1-[(1R)-3-(6-{[(BENZYLAMINO)CARBONYL]AMINO}-1H-INDOL-1-YL)-1-(HYDROXYMETHYL)PROPYL]-1H-IMIDAZOLE-4-CARBOXAMIDE | C24 H26 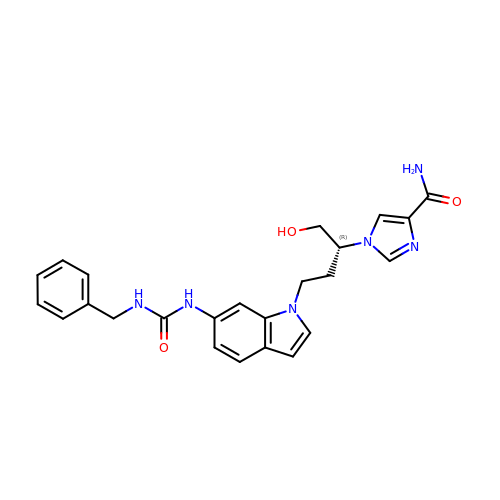N6 O3 | KCCUBLLGAMGDJL-HXUWFJFHSA-N>[3x]MKHHHHHHSAGLEVLFQGPMVLSPYKLNLVATPLFLK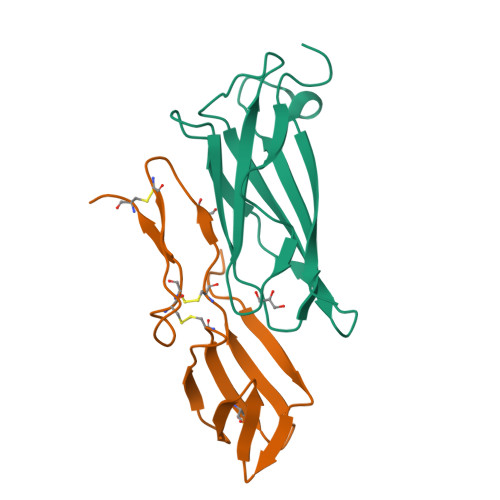PGIPYPIKVQVKDSLDQLVGGVPVTLNAQTIDVNQETSDLDPSKSVTRVDDGVASFVLNLPSGVTVLEFNVKTDAPDLPEENQAREGYRAIAYSSL;>MKHHHHHHSAGLEVLFQGPMGDVQERGHTYVTKNVTVEDGACVYLRNVIPNGETKALNNPCVLSTCYAADRKVNSTLCPNIGVDEGCHVEWTPDGVYPNCCPKHVCPSATASS[3x]> GSHMSKTLQRNRKMAMGRKKFNMDPKKGIQFLVENELLQNTPEEIARFLYKGEGLNKTAIGDYLGEREELNLAVLHAFVDLHEFTDLNLVQALRQFLWSFRLPGEAQKIDRMMEAFAQRYCLCNPGVFQSTDTCYVLSFAVIMLNTSLHN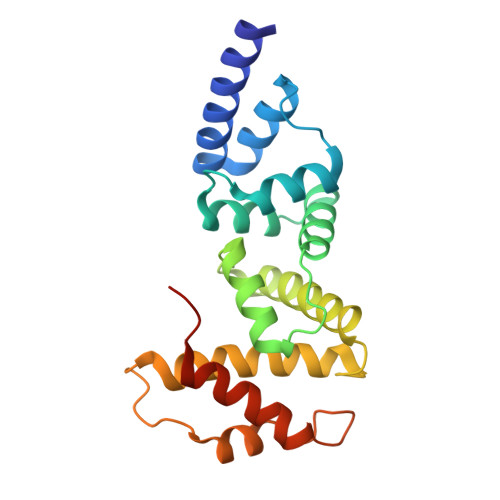PNVRDKPGLERFVAMNRGINEGGDLPEELLRNLYDSIRNEPFKIPEDDGN>GAAFTESQLMDEVPKKKFTGRCRLF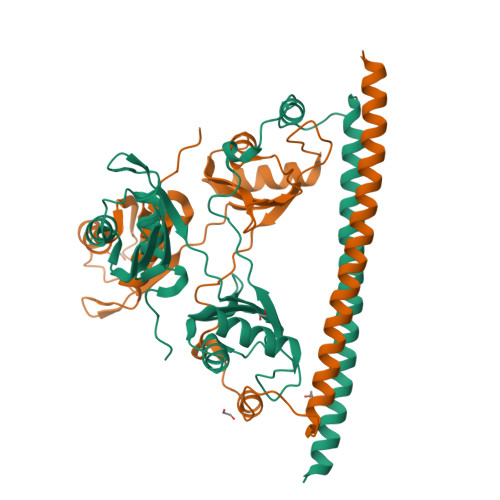VGNLPNEVKETELKELFSPHGDIAECYLSGKGFAFLRLDTRAHAESAKEAIDGRIIHGRQVRVRFAVHGAAIRVKELSPTVSNEMLYHAFSHFGDVERAVHIVDEKGRPTGEGIVEFERKPNCNEAMAAIRDKVFLLTASPKPLICEVLEPRDEDDGLAERMIPRTPGLSKERELGPRFPTPNSFEYVYGMKWKELYVVEQKRRAQLDEELRESRRRLESDMELAYQDYQAQML[2x]>MDIKELHVKTVKRGENVTMECSMSKVTNKDNLAWYRQSFGKVPQYFVRYYSSNSGYKFAEGFKDSRFSMTVNDQKFDLNII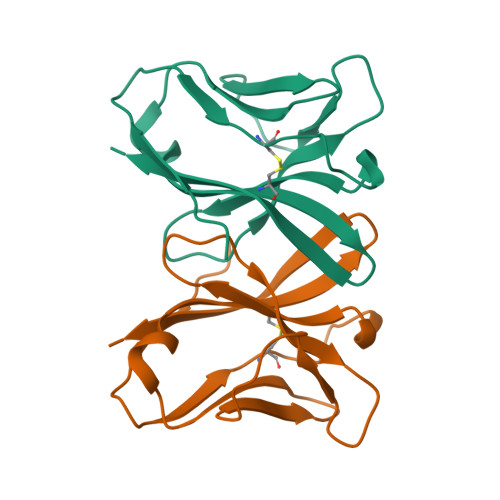GAREDDGGEYFCGEVEGIIIKFTSGTRLQF[4x]> MCDKSKTVLDYTIEFLDKYIPEWFETGNKCPLFIFFSGPQGSGKSFTSIQIYNHLMEKYGGEKSIGYASID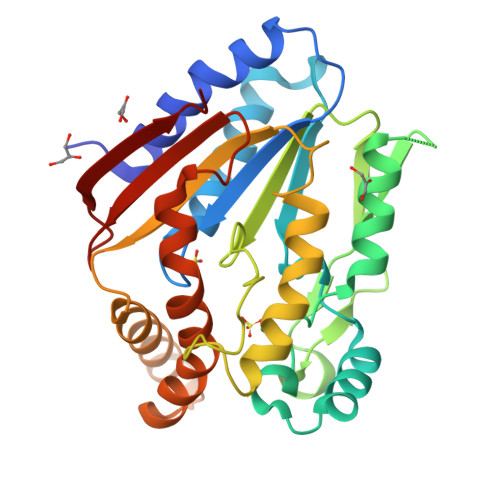DFYLTHEDQLKLNEQFKNNKLLQGRGLPGTHDMKLLQEVLNTIFNNNEHPDQDTVVLPKYDKSQFKGEGDRCPTGQKIKLPVDIFILEGWFLGFNPILQGIENNDLLTGDMVDVNAKLFFYSDLLWRNPEIKSLGIVFTTDNINNVYGWRLQQEHELISKVGKGMTDEQVHAFVDRYMPSYKLYLNDFVRSESLGSIATLTLGIDSNRNVYSTKTRCIE> AHHHERLRLRRDFLLIFKEGKSLQNEYFVVLFRKNGLDYSRLGIVVKRKFGKATRRNKLKRWVREIFRRNKGVIPKGFDIVVIPRKKLSEEFERVDFWTVREKLLNLLKRIEG

The focus of this work is Ribonuclease P (RNase P), the only ribozyme other than the ribosome that is present in all three domains of life (see for some reviews). While in archaea and eukaryotes, RNase P is comprised of one RNA subunit and four to ten proteins, in bacteria, this complex is formed by an RNA subunit (P RNA, 350–400 nucleotides, 110–125 kDa) and a single protein (P protein, ∼110 amino acids, 13 kDa). In all species, the P RNA serves as the primary biocatalyst for the cleavage of the 5′-leader sequence of pre-tRNAs during tRNA maturation. The P protein, on the other hand, binds the distal 5′-leader region of the pre-tRNA substrate, enhances the affinity of metal ions, and assists in product release.

Furthermore, purpurin, a competitive inhibitor which behaved as the most consistent hit across our assays, was shown to bind the P protein by X-ray crystallography, with its binding site corresponding to part of the 5′-leader binding site. We next determined that purpurin binds to the P protein with micromolar affinity in a dose-response relationship. Finally, the crystal structure of T. maritima P protein in complex with purpurin (DSupplementary Figure S21 and Table S2) shows a binding region of the compound located in a hydrophobic patch formed by residues Val 33, Leu 35 and Ile 87. Additional hydrogen-bonding interactions are observed between purpurin and Gln 28 and Arg 89. Arg 89 is a conserved protein residue, essential for efficient T. maritima RNase P activity, that potentially contacts the pre-tRNA leader binding region. Taken together, the binding and X-ray crystallography results indicate the existence of a region in the P protein that is sensitive to the binding of inhibitory compounds of T. maritima RNase P and that this region is also crucial for substrate binding. Remarkably, purpurin interferes with the binding of the leader to the P protein. Nonetheless, we succeeded in obtaining the crystal structure of the P protein in complex with purpurin, which binds in a region important for the 5′-leader interaction with the protein. This region includes R89, a highly conserved residue that makes putative contacts with the phosphate backbone of N-5 of the pre-tRNA leader. On the other hand, several lines of evidence point to purpurin as a potential inhibitor amenable to further optimization. This compound maintains inhibition even at remarkably high concentrations of MgCl2 (100 mM) and ammonium acetate (400 mM), shows a dose–response relationship in binding the holoenzyme, binding P protein and displacing pre-tRNA, and it presents a specific binding site on the P protein, as revealed by the co-crystal structure.>[6x]RGSHHHHHHGSFTPSGTTGTTKLTVTEKCQVRVGDLTVAKTRGQLTDAAPIGPVTVQALGCDA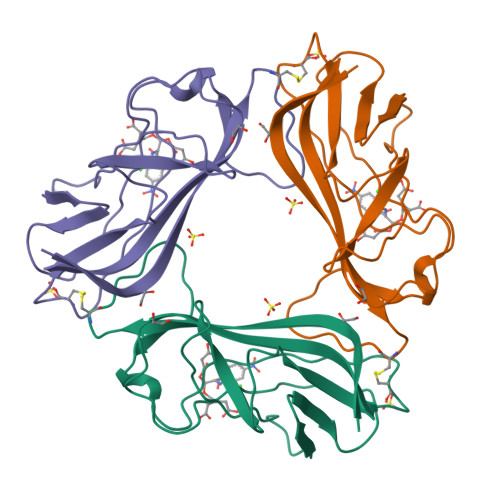RQVALKADTDNFEQGKFFLISDNNRDKLYVNIRPTDNSAWTTDNGVFYKNDVGSWGGIIGIYVDGQQTNTPPGNYTLTLTGGYWAK> MGSSHHHHHHSQENLYFQSQLTTRSKAIASKTK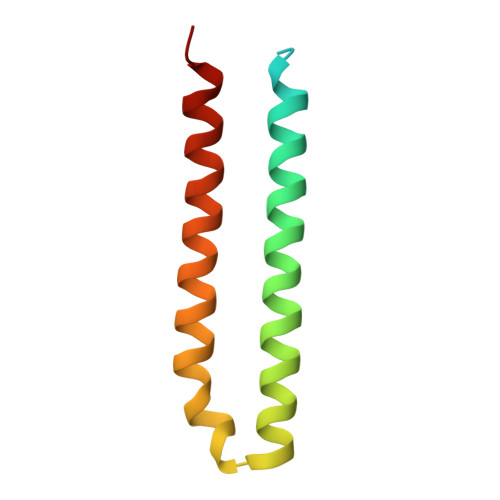EIEQVYRQDCETFGMVVKMLIEKDPSLEKSIQFALRQNLHEIGERCVEELKHFIAEYDTST>GAMASLVVPNLMGNKDKAD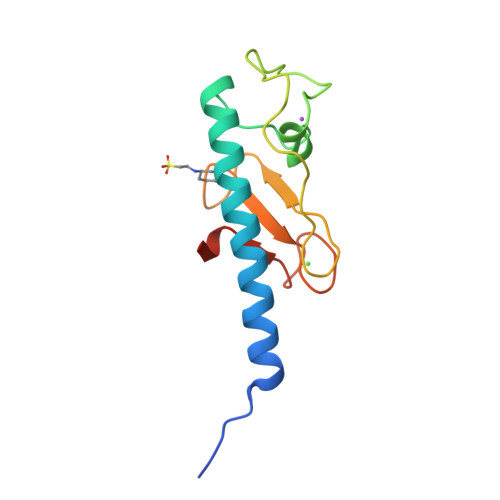RQKVMSDLVALESTLDMYRLDNNRYPTTEQGLRALVSKPTVQPEPRNYRQDGYIRRLPQDPWGGDYQLLNPGQYSDIDIFSPGPDGVPNTEDDIGNWTLGNAQP[2x]>[2x]PKIVVVGAVAGGA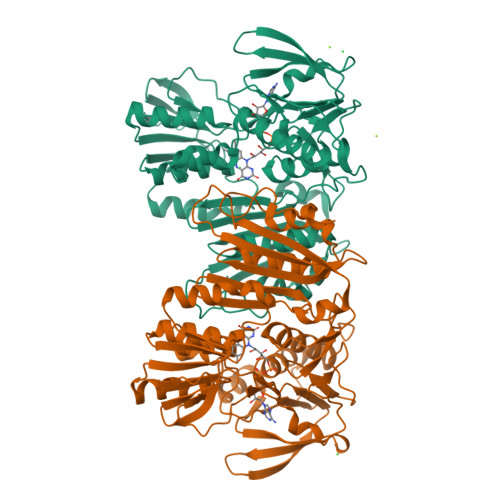TCASQIRRLDKESDIIIFEKDRDMSFANSALPYVIGEVVEDRRYALAYTPEKFYDRKQITVKTYHEVIAINDERQTVSVLNRKTNEQFEESYDKLILSPGASANSLGFESDITFTLRNLEDTDAIDQFIKANQVDKVLVVGAGYVSLEVLENLYERGLHPTLIHRSDKINKLMDADMNQPILDELDKREIPYRLNEEINAINGNEITFKSGKVEHYDMIIEGVGTHPNSKFIESSNIKLDRKGFIPVNDKFETNVPNIYAIGDIATSHYRHVDLPASVPLAWGAHRAASIVAEQIAGNDTIEFKGFLGNNIVKFFDYTFASVGVKPNELKQFDYKMVEVTQGAHANYYPGNSPLHLRVYYDTSNRQILRAAAVGKEGADKRIDVLSMAMMNQLTVDELTEFEVAYAPPYSHPKDLINMIGYKAK> MHHHHHHMSDLDRLASRAAIQDLYSDQLIGVDKRQEGRLASIWWDDAEWTVEGIGTYKGPEGALDLVNNVVWPRWHDFIHYGTNLR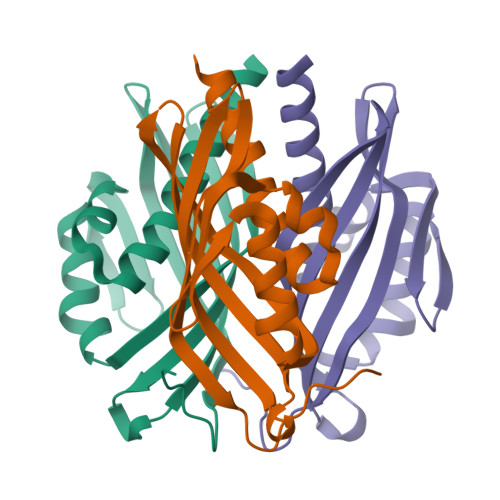LEFVSADKVNGIGDVLCLGNLVEGNQSILIAAVYTSEYERRDGVWKFSKLNGRMNYFTPLAGIHFVPPGA>[2x]SPSPLNPGTNVARLAEQAPIHWVSVAQIENSLAGRPPMAVGFDIDDTVLFSSPGFWRGKKTFSPESEDYLKNPVFWEKMNNGWDEFSIPKEVARQLIDMHVRRGDAIFFVTG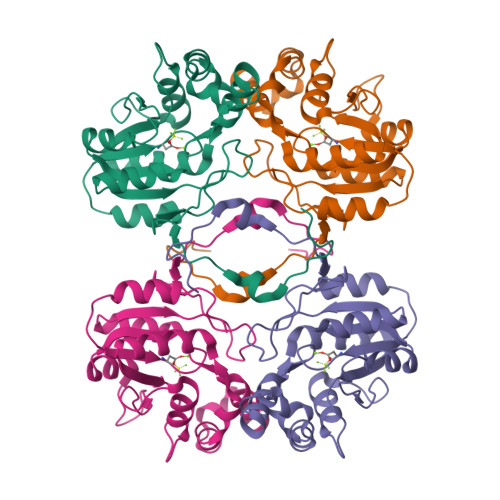RSPTKTETVSKTLADNFHIPATNMNPVIFAGDKPGQNTKSQWLQDKNIRIFYGDSDNDITAARDVGARGIRILRASNSTYKPLPQAGAFGEEVIVNSEY> MFNRNFILRAAEFKQKSRWSSVWPNMRYGSMFLSYSVGRKLPMKGVNWVTRDSNRLLNFSNRYSAVISDIDVKRTEEELNVALSDIRWNDHRRIYWKCSFCGSSYRKNVSVRTKYHAGCNFCKKKYPSEVRGEQHGSPPVSQAAPELTEQLV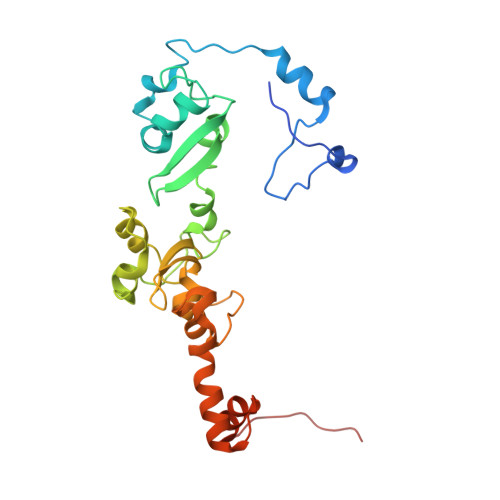DNGKRDNLATLAVTSKFYAEWTCRGCGGSYRSTIRSRTGQVEAGQCTLHPDIVAWSAYCPSCSWRPNMVPIAEEVSRSGQFLGLERSMEELGGQRGKQLPIPRRKRLAC>MAKEFGIPAAVAGTVLNVVEAGGWVTTIVS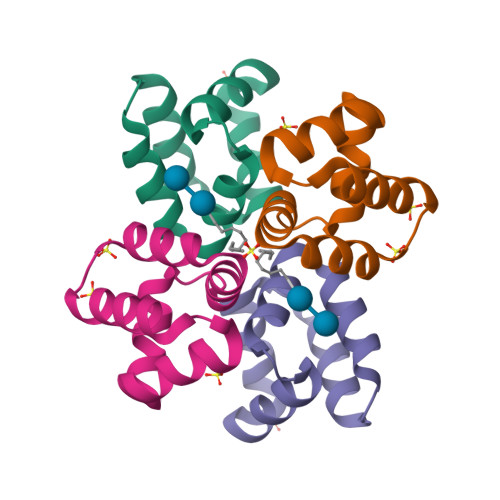ILTAVGSGGLSLLAAAGRESIKAYLKKEIKKKGKRAVIAW[2x]> NVKKFPEGFLWGAATSSYQIEGAWNEDGKGESIWDRFTRIPGKIKNGDSGDVACDHYHRYEQDLDLMRQLGLKTYRFSIAWARIQPDSSRQINQRGLDFYRRLVEGLHKRD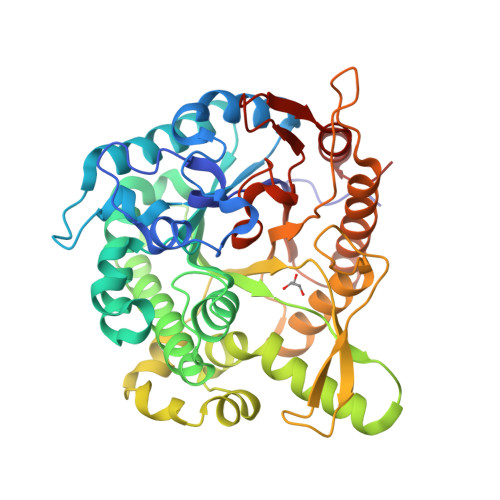ILPMATLYHWDLPQWVEDEGGWLSRESASRFAEYTHALVAALGDQIPLWVTHNEPMVTVWAGYHMGLFAPGLKDPTLGGRVAHHLLLSHGQALQAFRALSPAGSQMGITLNFNTIYPVSAEPADVEAARRMHSFQNELFLEPLIRGQYNQATLMAYPNLPEFIAPEDMQTISAPIDFLGVNYYNPMRVKSSPQPPGIEVVQVESPVTAMGWEIAPEGLYDLLMGITRTYGKLPIYITENGAAFDDQPDQSGQVNDPQRVGYFQGHIGAARRALADGVDLRGYYAWSLLDNFEWAEGYSKRFGIIYVDFETQQRTLKQSAQWYRDVIANNGLED> MLRKFHVVGISTRIVVNTFGDHNPNGRIYVLKENESKLKDLVRKNPYKPIDLVQPLAIRANEGDIVEILFENQLSFSAGMHFQEADYSVLSSDGADAGYNPDTTVEPGGEILYRLNVNQEGICFFTDLGNVSSTEQGSSVQGLFGALLVQKRGSSWTDPVTGGPINSGVYADIHHPFLPSFREYAWFFNDEMEIRDLTGERPLNPMTNQEAESFHGVNLRYEPMTNRKRLMEAGVVCPDCDSEEVHHDSWVFGDPATPILRGYVGDPAVIRLIHGGVKETHVFHYHVHQWLGDSSNINAEILDAQSISPQTHYSIQPLYGLGSLHGAIGDSIIHCHLYPAFGIGMWGMNRVFDTLQDGSQCYPNGVRIKALMPLPDRPEPPKPTPEKPGFPNFIPGKVGYKAPRPPLGIVGGREMTELERNAAIENPRPGAVFVDPCLDQDPVVVEFNVSAIEMPVVYNKQGWHDPKARFYVMDEDLDDILSGKKEPEPLVFHVPAGTCIRMNYTNRMPHILDGDAFQLVTRTYENGFHIHFVKFDVLACDGGNVGWNYDSAVLPGQTIRYEWYAETELKAFFFHDHLFANSHQQHGVFGAGVIQPRFSKFLDSRTGDEVDHGTQISVEHPLIPDYRDQTLFVHDFALLFDKNGRPIQPPEYPGSEDDPGVFGVNFKCEPLKFRLGEDCDPAYSFSSYVHGDPVTPILRAYEGDPIRIRLLQGAHEESHSFNIHGLRWKEERPDLGSSMKAQQHIGISESFTFETEIPASGDYLWAFEDEEDVWLGTWGLIRAYKGRMEDLIVLTDREALPEGSAETPKPTGKPPEKANPLASLPPGAYQGSPVKKFEVVAFQTPIQYNSYGDHDPYGIIFALKEDVEDILTGKKNPVPLILRANVGDLVEVTLTSELKKELFPFQDGIHPYPPVKEQSFYPPSLRISLHTSLLNYDVKTS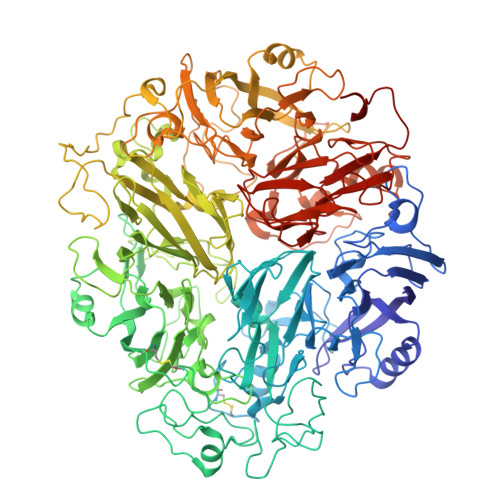SGDTVGYNPDQTVGPGETITYRWFVDGQFGMCSMWDMADLRNHRSFGTFGAFVAESRFTTYLDPYSLEKAITGENVILRHPLLPATREFVLILHDGVRLEDKDGKVIIDPMDGVVPDTEELEEVDTYDYGSRGFNYRSERLINRYKEHPVMHELFSSEVFGDPATPLFEAYPGEPVVMRITTPAERRRAHTFHLHGHYWKFDSKDLDSRIQSFLGHMVTGHTDDLRLIGGAGGVFNFPGDYLYRSGNIRWDIELGMWGIFRVHKDSKENLPRLEEVEGGWDNEEKA> VDPTHFEKRFLKRIRDLGEGHFGKVELCRYDPEGDNTGEQVAVKSLKPESGGNHIADLKKEIEILRNLYHENIVKYKGICTEDGGNGIKLIMEFLPSGSLKEYLPKNKNKINLKQQLKYAVQICKGMDYLGSRQYVHRDLAARNVLVESEHQVKIGDFGLTKAIETDKEYYTVKDD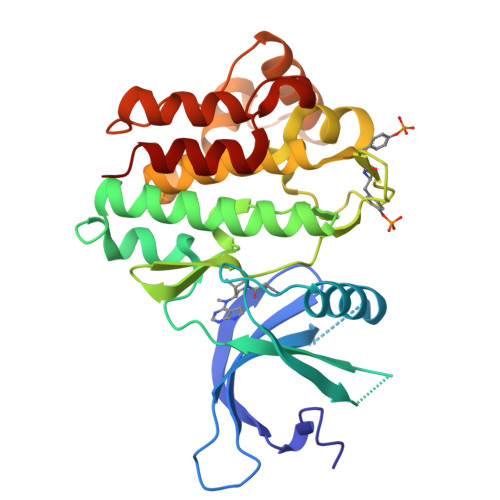RDSPVFWYAPECLMQSKFYIASDVWSFGVTLHELLTYCDSDSSPMALFLKMIGPTHGQMTVTRLVNTLKEGKRLPCPPNCPDEVYQLMRKCWEFQPSNRTSFQNLIEGFEALLK>MLESNENRIQIMSTIAKIYRAMSRELN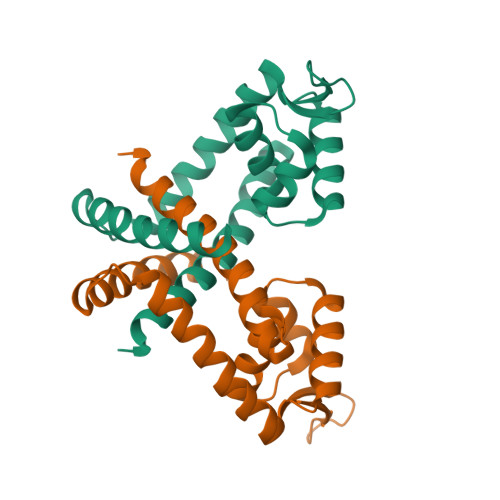RRLGELNLSYLDFLVLRATSDGPKTMAYLANRYFVTQSAITASVDKLEEMGLVVRVRDREDRRKILIEITEKGLETFNKGIEIYKKLANEVTGDLSEDEVILVLDKISKILKRIEEISQ[2x]>MIYSITEIEARYAETDKMGVIYHG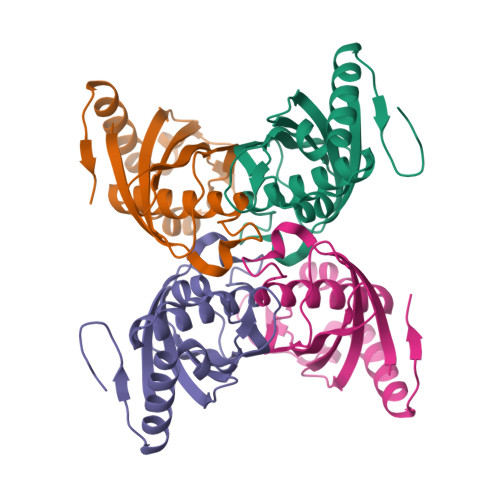NYATWFEVARLDYISKLGFSYADMEKQGIISPVTDLNVNYKKSIFYPEKVKVKTWVEKYSRLRSVYKYEIFNEKGELATTGSTELICIKEDTFKPIRLDRYFPDWHEAYSKVQALNNEGKIVEIMDGIDSL[4x]> SSDFVRKLYKMLEDPSYHSVVRWSDDGDSFVVLENEKFTKTILPKHFKHSNFASFVRQLNKYDFHKVRHNDENGESPYGRDAWEFKHPEFRADRKDNLDNI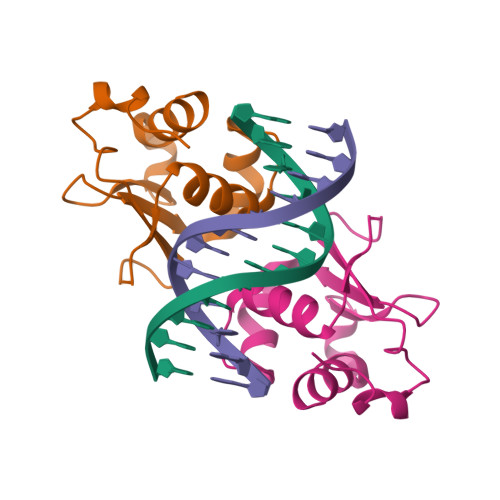RRK>[4x]MVIATDDLETTCPNCNGSGREEPEPCPKCLGKGVILTAQGSTLLHFIKKHIHE

In Bacillus subtilis tryptophan biosynthesis is regulated by two proteins, the trp RNA-binding attenuation protein (TRAP) and Anti-TRAP (AT), which are involved in sensing levels of free tryptophan and uncharged tryptophanyl transfer RNA (tRNATrp), respectively. AT antagonises TRAP action by binding to tryptophan-activated TRAP and preventing its interaction with the leader region of the trp mRNA. Binding of zinc ion is essential for formation of AT oligomers and for its function. Here, we report two crystal structures of Bacillus licheniformis AT, which shares 66% sequence identity with B. subtilis AT.

The low-pH crystals belong to the space group H3 with four AT monomers per asymmetric unit whereas the high-pH crystals belong to the space group P21 and contain 48 AT monomers in the asymmetric part. Packing of the trimer and the additional AT subunit around the crystallographic 3-fold axis generates four AT trimers that form a dodecameric particle. The architecture of this dodecamer is identical to the one observed for B. subtilis AT at pH 6.5. As with B. subtilis AT, trimer–trimer association within the B. licheniformis dodecamer is maintained mainly by hydrophobic interactions in two regions. The first is a hydrophobic area in the centre of the molecule, lined by residues 1–3 from all 12 AT monomers. The second region of stabilising interactions includes van der Waals contacts between pairs of adjacent zinc-binding domains formed along the 2-fold molecular axes by residues Pro13 and Ile35. An interesting feature of the low-pH dodecamer is the relatively large internal chamber inside the multimeric assembly, which is centred at the intersection of symmetry axes and is isolated from the solvent. There are no peaks in the electron density maps inside the chamber suggesting that it is filled by disordered crystallisation buffer components or solvent. Its inner surface is lined by the side chains of twelve Val2 residues, this amino acid is strictly conserved in AT proteins. The chamber could be fitted with a sphere of ∼11 Å in diameter, potentially permitting the accommodation of a relatively large ligand. The calculated pKa value for the amino group of Met1 is 7.1. This indicates that the salt bridge formation is favoured in case of the low-pH crystal form (pH 6.0) as the amino group of Met1 is likely to be protonated.> MIFPKQYPIINFTTAGATVQSYTNFIRAVRGRLTVLPNCVGLPINQRFILVELSNHAELSVTLALDVCNAYVVGYRAGNSAYFFHPDNQEDAEAITHLFTDVQNRYTFAFGGNYDRLEQLAGNLRENIELGN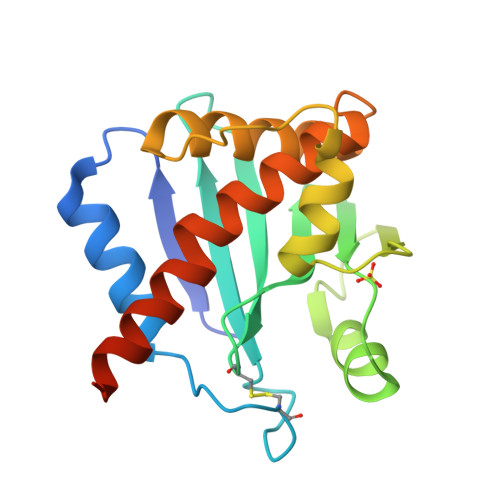GPLEEAISALYYYSTGGTQLPTLARSFIICIQMISEAARFQYIEGEMRTRIRYNRRS>[12x]AEIYNKDGNKVDLYGKAVGLHYFSKGNGENSYGGNGDMTYARLGFKGETQINSDLTGYGQWEYNFQGNNSEGADAQTGNKTRLAFAGLKYADVGSFDYGRNYGVVYDALGYTDMLPEFGGDTAYSDDFFVGRVGGVATYRNSNFFGLVDGLNFAVQYLGKNERDTARRSNGDGVGGSISYEYEGFGI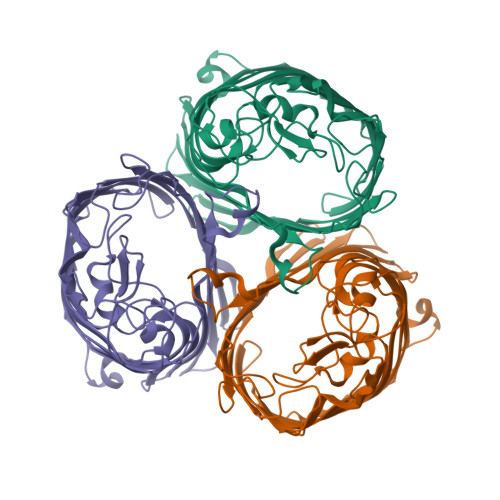VGAYGAADRTNLQEAQPLGNGKKAEQWATGLKYDANNIYLAANYGETRNATPITNKFTNTSGFANKTQDVLLVAQYQFDFGLRPSIAYTKSKAKDVEGIGDVDLVNYFEVGATYYFNKNMSTYVDYIINQIDSDNKLGVGSDDTVAVGIVYQF> MRLSYEALEWRTPIENSTEPVSLPPPPPFFGQERAREALELAIRGGFHAYLVGPPSLGKHEALLAYLSTQSVETPPDLLYVPLSERKVAVLTLPSGQEIHLAEAVEGLLLEVNRLDELFRQGSFLREKTQLEARFKEAREQQLEALRREAQEAGFALSTNGERLELTGPGPVPAELSARLEEVTLGSLAASAELEVALRRLRRDWALHYLNNRFEPLFQRFPQARAYLEALRARLARYAETGEPLDPAQWRPNLLTSSSSGTPPPIVYEPYATAPRLFGRLDYLVDRGVWSTNVSLIRPGAVHRAQGGYLILDALSLKREGTWEAFKRALRNGQVEPVTEPQAPAGLEVEPFPIQMQVILVGTPEAFEGLEEDPAFSELFRIRAEFSPTLPASPENCTALGGWLLAQGFQLTQGGLTRLYDEARRMAEQRDRMDARLVEIRALAEEAAVLGGGLL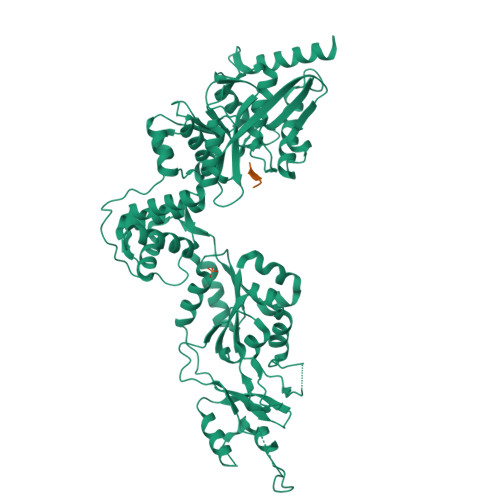TAESVEQAIAAREHRSFLSEEEFLRAVQEGVIRLRTTGRAVGEVNSLVVVEAAPYWGRPARLTARAAPGRDHLISIDREAGLGGQIFHKAVLTLAGYLRSRYIEHGSLPVTISLAFEQNYVSIEGDAAGLAELVAALSAIGNLPLRQDLAVTGAVDQTGKVLAVGAINAKVEGFFRVCKALGLSGTQGVILPEANLANLTLRAEVLEAVRAGQFHIYAVETAEQALEILAGARMEGFRGLQEKIRAGLEAFARLEEGHDKEDREKLAAALEHHHHHH;> APEAV> MRNQGLGSWPVRRARMSPHATAVRHGGTALTYAELSRRVARLAHGLREAGVRPGDRVAYLGPNHPAYLETLFACGQAGAVFVPLNFRLGVPELDHALADSGASVLIHTPEHAETVAALAGDRLLRVPAGELEAADDEPLDLPVGLDDVCLLMYTSGSTGRPKGAMLTHGNLTWNCVNVLVETDLASDERALVAAPLFHAAALGMVCLPTLLKGGTVILHSAFDPGAVLSAVEQERVTLVFGVPTMYQAIAAHPRWRSTDLSSLRTLLCGGAPVPADLAGRYLDRGLAFVQGYGMTEAAPGVLVLDRAHVAEKIGSAGVPSFFTDVRVAGPSGEPVPPGEKGEIVVSGPNVMKGYWGRPEATAEVLRDGWFRSGDVATVDGDGYFHVVDRLKDMIISGGENIYPAEVENELYGYPGVEACAVIGVPDPRWGEVGKAVVVPAAGSRIDGAELLAWLRTRLAGYKVPKSVEFTDRL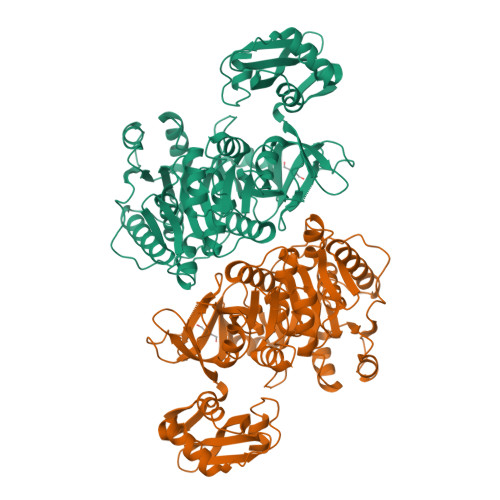PTTGSGKILKGEVRRRFGLEHHHHHH>RTKDKYRVVYTDHQRLELEKEFHYSRYITIRR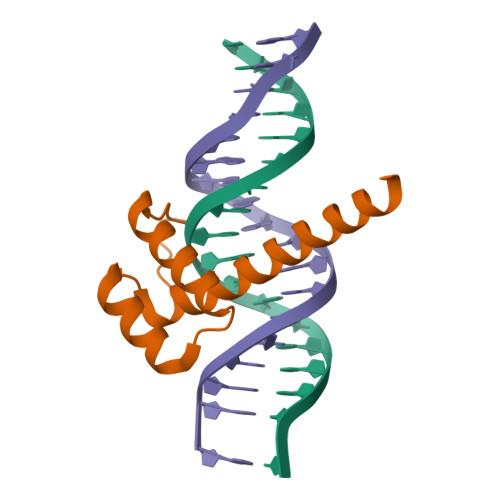KAELAATLGLSERQVKIWFQNRRAKERKINKKKLQQQQQQ[2x]> MSADSSPLVGSTPTGYGTLTIGTSIDPLSSSVSSVRLSGYC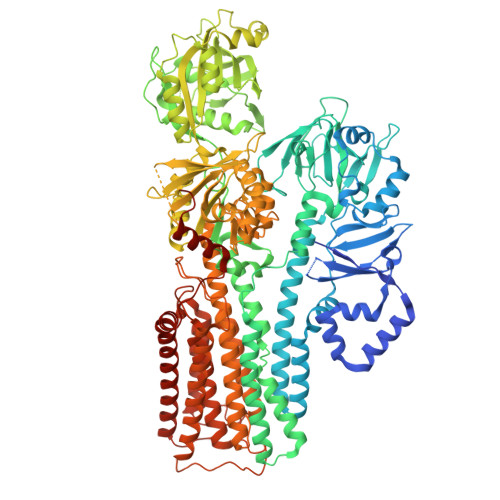GSPWRVIGYHVVVWMMAGIPLLLFRWKPLWGVRLRLRPCNLAHAETLVIEIRDKEDSSWQLFTVQVQTEAIGEGSLEPSPQSQAEDGRSQAAVGAVPEGAWKDTAQLHKSEEAKRVLRYYLFQGQRYIWIETQQAFYQVSLLDHGRSCDDVHRSRHGLSLQDQMVRKAIYGPNVISIPVKSYPQLLVDEALNPYYGFQAFSIALWLADHYYWYALCIFLISSISICLSLYKTRKQSQTLRDMVKLSMRVCVCRPGGEEEWVDSSELVPGDCLVLPQEGGLMPCDAALVAGECMVNESSLTGESIPVLKTALPEGLGPYCAETHRRHTLFCGTLILQARAYVGPHVLAVVTRTGFCTAKGGLVSSILHPRPINFKFYKHSMKFVAALSVLALLGTIYSIFILYRNRVPLNEIVIRALNLVTVVVPPALPAAMTVCTLYAQSRLRRQGIFCIHPLRINLGGKLQLVCFDKTGTLTEDGLDVMGVVPLKGQAFLPLVPEPRRLPVGPLLRALATCHALSRLQDTPVGDPMDLKMVESTGWVLEEEPAADSAFGTQVLAVMRPPLWEPQLQAMEEPPVPVSVLHRFPFSSALQRMSVVVAWPGATQPEAYVKGSPELVAGLCNPETVPTDFAQMLQSYTAAGYRVVALASKPLPTVPSLEAAQQLTRDTVEGDLSLLGLLVMRNLLKPQTTPVIQALRRTRIRAVMVTGDNLQTAVTVARGCGMVAPQEHLIIVHATHPERGQPASLEFLPMESPTAVNGVKDPDQAASYTVEPDPRSRHLALSGPTFGIIVKHFPKLLPKVLVQGTVFARMAPEQKTELVCELQKLQYCVGMCGDGANDCGALKAADVGISLSQAEASVVSPFTSSMASIECVPMVIREGRCSLDTSFSVFKYMALYSLTQFISVLILYTINTNLGDLQFLAINLVITTTVAVLMSRTGPALVLGRVRPPGALLSVPVLSSLLLQMVLVTGVQLGGYFLTLAQPWFVPLNRTVAAPDNLPNYENTVVFSLSSFQYLILAAAVSKGAPFRRPLYTNVPFLVALALLSSVLVGLVLVPGLLQGPLALRNITDTGFKLLLLGLVTLNFVGAFMLESVLDQCLPACLRRLRPKRASKKRFKQLERELAEQPWPPLPAGPLR>[5x]GAMADREKLLTESGVYGTFATFQMDHDW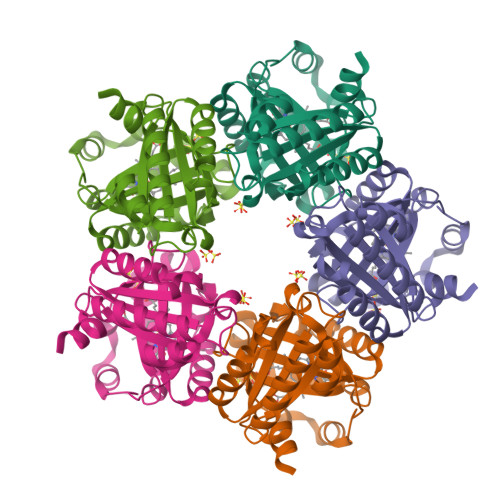WDLPGESRVISVAEVKGLVEQWSGKILVESYLLRGLSDHADLMFRVHARTLSDTQQFLSAFMGTRLGRHLTSGGLLHGVSKKPTYVAGFPESMKTELQVNGESGSRPYAIVIPIKKDAEWWALDQEARTALMQEHTQAALPYLKTVKAKLYHSTGLDDVDFITYFETERLEDFHNLVRALQQVKEFRHNRRFGHPTLLGTMSPLDEILEKFAQ> MGLTGLEIYKHLPKKNCKECGQPTCLAFAMQIAAGKAGLDACPYVSDEAKELLESASAPPVALIKVGKGEKVLEIGHETVLFRHDKRFEHPCGLAILVEDTLSEGEIKERVEKINKLVFDRVGQMHSVNLVALKGSSQDAATFAKAVATAREVTDLPFILIGTPEQLAAALETEGANNPLLYAATADNYEQMVELAKKYNVPLTVSAKGLDALAELVQKITALGYKNLILDPQPENISEGLFYQTQIRRLAIKKLFRPFGYPTIAFALDENPYQAVMEASVYIAKYAGIIVLNTVEPADILPLITLRLNIYTDPQKPIAVEPKVYEILNPGPDAPVFITTNFSLTYFCVAGDVEGARIPAYILPVDTDGTSVLTAWAAGKFTPEKIAQFLKESGIAEKVNHRKAILPGGVAVLSGKLQELSGWEI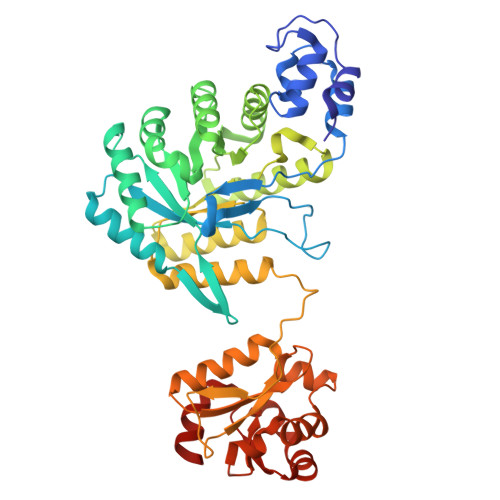LVGPRESSGINSFIKQRWNV>[2x]QDKGSVGIAMPTKSSARWIDDGNNIVKQLQEAGYKTDLQYADDDIPNQLSQIENMVTKGVKVLVIASIDGTTLSDVLKQAGEQGIKVIAYDRLIRNSGDVSYYATFDNFQVGVLQATSITDKLGLKDGKGPFNIELFGGSPDDNNAFFFYDGAMSVLKPYIDSGKLVVKSGQMGMDKVGTLRWDPATAQARMDNLLSAYYTD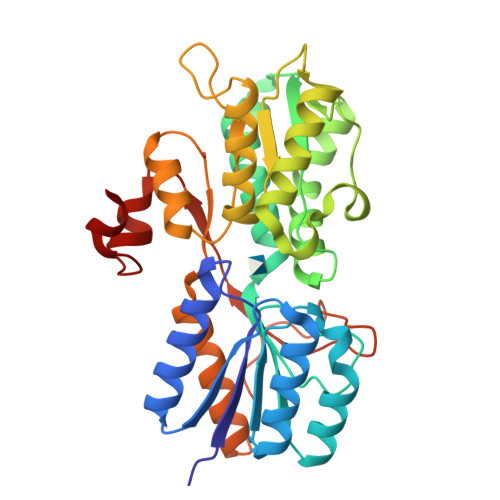AKVDAVLSPYDGLSIGIISSLKGVGYGTKDQPLPVVSGQDAEVPSVKSIIAGEQYSTIFKDTRELAKVTVNMVNAVMEGKEPEVNDTKTYENGVKVVPSYLLKPVAVTKENYKQVLVDGGYYKEDQLK>[4x]MASGMIVTDAGADQP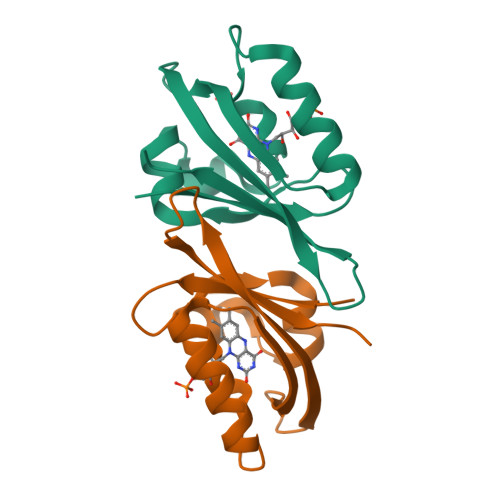IVFVNRAFSTITGYAPNEVLGRNARFLQGPQTDAATVARLREAIAAARPIQERILNYRKDGQPFWNQLSISPVRDETGNVVAFVGVKTDVTAHHHHHH>[4x]SNAMIKQRTLKNIIRATGVGLHSGEKVYLTLKPAPVDTGIVFSRTDLDPVVEIPARAENVGETTMSTTLVKGDVKVDTVEHLLSA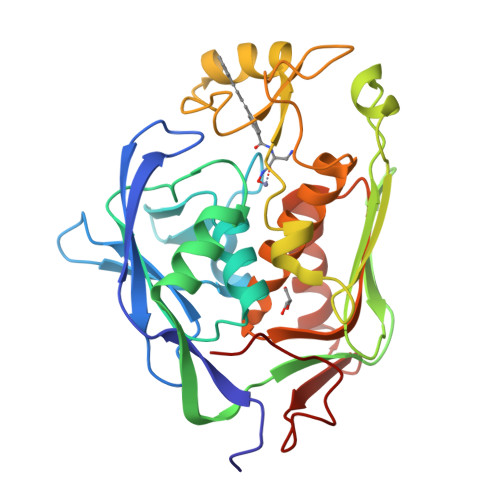MAGLGIDNAYVELSASEVPIMDGSAGPFVFLIQSAGLQEQEAAKKFIRIKREVSVEEGDKRAVFVPFDGFKVSFEIDFDHPVFRGRTQQASVDFSSTSFVKEVSRARTFGFMRDIEYLRSQNLALGGSVENAIVVDENRVLNEDGLRYEDEFVKHKILDAIGDLYLLGNSLIGEFRGFKSGHALNNQLLRTLIADKDAWEVVTFEDARTAPISYMRP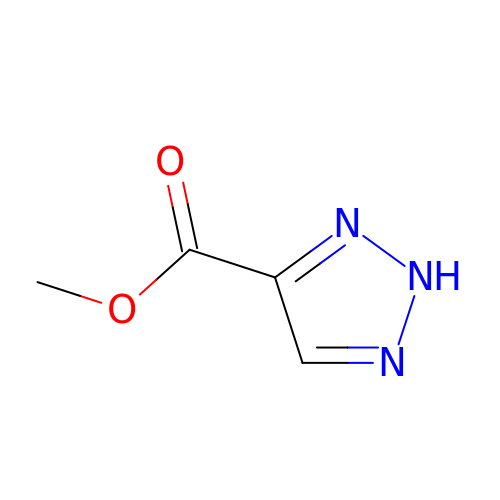METHYL 2H-1,2,3-TRIAZOLE-4-CARBOXYLATE | C4 H5 N3 O2 | FZXQUCUWEZQIHL-UHFFFAOYSA-N>MALVKIVRIETFPLFHRLEKPYGDANGFKRYRTCYLIRIITESGIDGWGECVDWLPALHVGFTKRIIPFLLGKQAGSRLSLVRTIQKWHQRAASAVSMALTEIAAKAADCSVCELWGGRYREEIPVYASFQSYSDSPQWISRSVSNVEAQLKKGFEQIKVKIGGTSFKEDVRHINALQHTAGSSITMILDANQSYDAAAAFKWERYFSEWTNIGWLEEPLPFDQPQDYAMLRSRLSVPVAGGENMKGPAQYVPLLSQRCLDI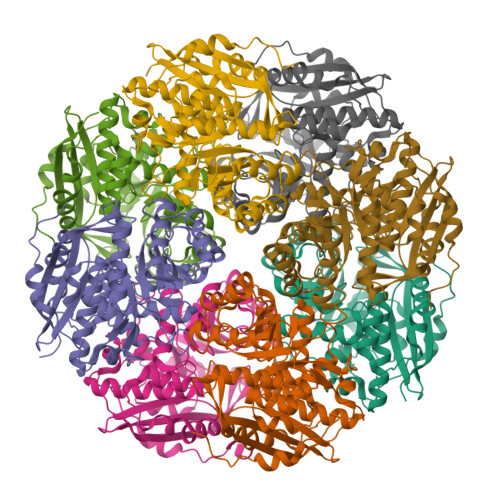IQPDVMHVNGIDEFRDCLQLARYFGVRASAHAYDGSLSRLYALFAQACLPPWSKMKNDHIEPIEWDVMENPFTDLVSLQPSKGMVHIPKGKGIGTEINMEIVNRYKWDGSAYEGHHHHHH[8x]>FDHCFKKSSDGFLYCEGTKVQDIMETVEKRPFYLYSKPQITRNLEAYKEALEGVRSVIGYAIKANNNLKILEHLRSLGCGAVLVSGNELRLALLAGFDPTKCIFNGNGKSLEDLVLAAQEGVFVNVDSEFDLNNIVEASRISGKQVNVLLRINPDVDPQVHPYVATGNKNSKFGIRNEKLQWFLDEVKAHPKELKLVGAHCHLGSTITKVDIFRDAAVLMIEYIDEIRRQGFEVSYLNIGGGLGIDY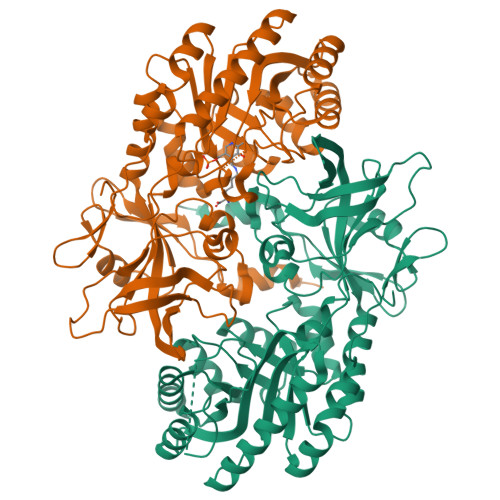YHAGAVLPTPMDLINTVRELVLSRDLNLIIEPGRSLIANTCCFVNHVTGVKTNGTKNFIVIDGSMAELIRPSLYDAYQHIELVSPTPPEAEVTKFDVVGPVCESADFLGKDRELPTPPQGAGLVVHDAGAYCMSMASTYNLKMRPPEYWVEEDGSITKIRHAETFDDHLRFFEGL[2x]> GGYVAPKAVWLPAV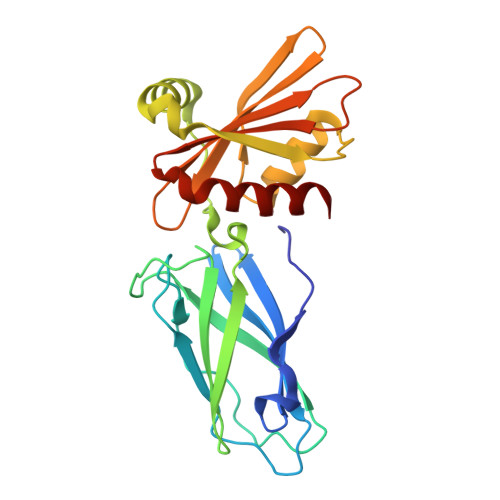KAKGLEISGTFTHRQGHIYMEMNFTNKALQHMTDFAIQFNKNSFGVIPSTPLAIHTPLMPNQSIDVSLPLNTLGPVMKMEPLNNLQVAVKNNIDVFYFSCLIPLNVLFVEDGKMERQVFLATWKDIPNENELQFQIKECHLNADTVSSKLQNNNVYTIAKRNVEGQDMLYQSLKLTNGIWILAELRIQPGNPNYTLSLKCRAPEVSQYIYQVYDSILKN> NAERGDADGGTSALRVTREQFHDGSRGLFRPHPFNRRFARVRKPVFPIEARNLRLMYKRKSKRRRGRGDKSNAKGIRWKHVHQQAGRYKGPRSRTFEGGKLPLYRRIPKWPDAWLARQRKVLEPLNLAKLRTFIESGRLDTRFTITQRHLNDSRCVKVKNGVSLFNVNDYPFPYKISIE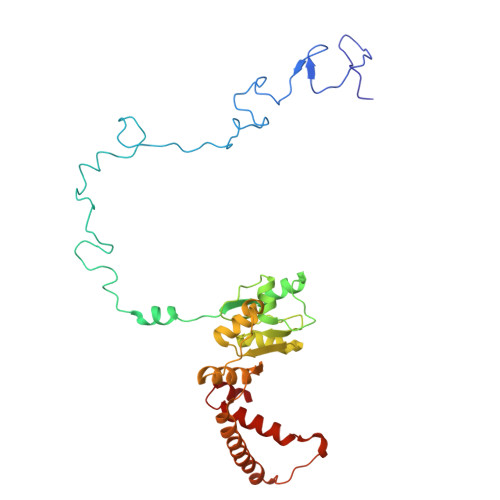VAGADQSSIDAIRRVGGEVIIVYRNRLNLRAHIKPYKFEVLPKTARPNLEMVHYLEKMRARGCVVKYVKPQWLIDEEKSLKTELAEFEAEALIAKGEAIERGDPDLRESVDDLQQRLLKRFRLRETRAAELL>[2x]MSDERYQQRQ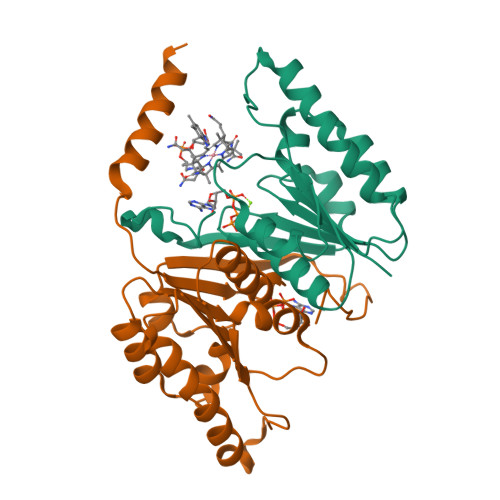QKVKDRVDARVAQAQEERGIIIVFTGNGKGKTTAAFGTAARAVGHGKNVGVVQFIKGTWPNGERNLLEPHGVEFQVMATGFTWETQNREADTAACMAVWQHGKRMLADPLLDMVVLDELTYMVAYDYLPLEEVISALNARPGHQTVIITGRGCHRDILDLADTVSELRPVKHAFDAGVKAQMGIDY> TTASATGIATLTSTGDVLDVWYPEIGSTDQSALTPLEGVDEDRNVTRKIVTTTIDIDAAPTDTYDAWLRLHLLSHRVFRPHTINLDGIFGLLNNVVWTNFGPCAVDGFALTRARLSRRGQVTVYSVDKFPRMVDYVVPSGVRIG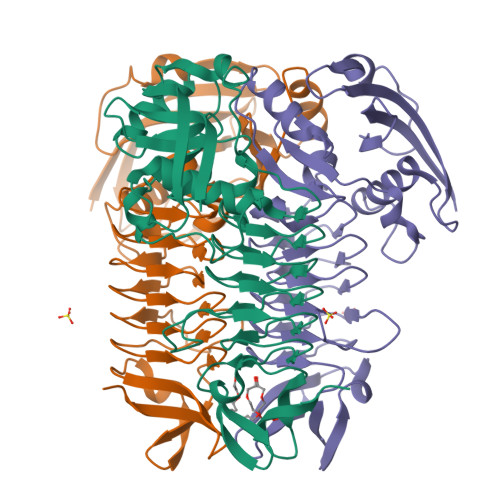DADRVRLGAYLADGTTVMHEGFVNFNAGTLGASMVEGRISAGVTVDDGTDVGGGASIMGTLSGGGQHVISLGKRCLLGANSGCGIPLGDDCIIEAGLYITAGTKVLFDGSLHKASTLAGSNGLIFRRDSVSGQVVAVPNTKVVELNTALHSNHHHHHH> G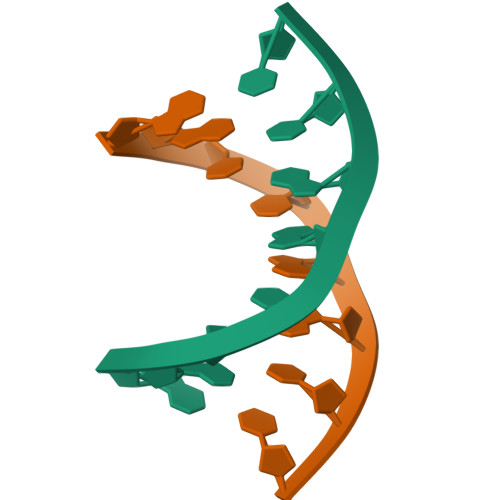GCCGGCC(2S)-7-amino-2-{[(R)-hydroxy{(1R)-2-methyl-1-[(3-phenylpropanoyl)amino]propyl}phosphoryl]methyl}heptanoic 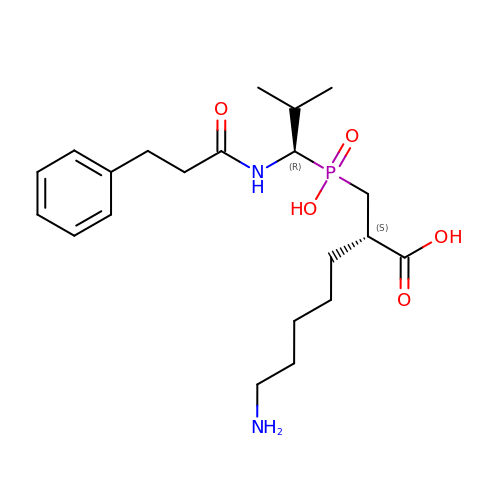acid | C21 H35 N2 O5 P | DEWOTLFUKYSXIE-UYAOXDASSA-N>[2x]GPLGSARRLYVGNIPFGITEEAMMDFFNAQMRLGGLTQAPGNPVLAVQINQDKNFAFLEFRSVDETTQAMAFDGIIFQGQSLKIRRPHVYQPLPGAHKLFIGGLPNYLNDDQVKELLTSF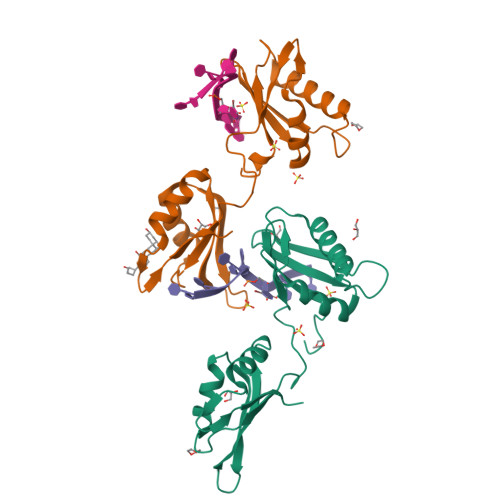GPLKAFNLVKDSATGLSKGYAFCEYVDINVTDQAIAGLNGMQLGDKKLLVQRAS The cadherin-catenin cell adhesion complex is the major building block of AJs, and has a crucial function in the dynamic behaviors of epithelial cells, such as cell polarization and cell rearrangements. The structure of α-catenin (100 kDa) consists of three distinct domains. The C-terminal actin-binding domain (ABD) (28 kDa), which is connected to the rest by a flexible P-linker region28 (2 kDa), directly binds to F-actin, and closely resembles the vinculin ABD (vin-ABD). The direct interaction between α-catenin and F-actin was demonstrated to be a catch bond, an interaction that is stabilized by increased force.

To better characterize the αE-catenin actin-binding site, we elucidated a crystal structure of αEcat-ABD-WT at 2.2-Å resolution. The electron density map of α5-helix clearly shows that V796 adopts a conformation that exposes its side chain on the ABD surface, along with two additional hydrophobic residues L785 and I792. Our observations of the cryptic (attenuated) and exposed (activated) conformations of V796, despite the nearly identical primary sequences of αEcat- and αNcat-ABDs (87% identity), indicate that this residue resides within a conformationally dynamic region. Consistent with this idea, the αEcat-ABD-WT structure contains an internal cavity that could accommodate V796 in the cryptic state similar to V796N in the αNcat-ABD-WT structure. This internal cavity is partly formed by the side chain of M673 from α1-helix, hence raising the possibility that α1-helix unfolding allosterically affects the F-actin-binding site by changing the conformational dynamics of V796. Our site-directed mutagenesis and actin cosedimentation assays with the αEcat-ABD variants support critical roles of these hydrophobic residues in F-actin-binding: Ala substitutions of L785, I792 and V796, individually or together as 3A, led to a range of reduction (75, 36, 47, and 78%, respectively) in the amount of ABD cosedimenting with F-actin compared to αEcat-ABD-WT. The equally significant reduction observed with either the L785A mutation alone or 3A suggests that L785 plays a central role in establishing the critical hydrophobic interface between F-actin and αcat-ABD. The measurable reduction in F-actin binding with I792A or V796A suggests that I792 and V796 are likely involved in further stabilizing this interface, and any changes to these residues could modulate the F-actin-binding activity of αcat-ABD. These results confirm that the hydrophobic residues on the α5-helix surface constitute an important binding surface for F-actin interaction.

>[2x]GPLGSPEFSRTSVQTEDDQLIAGQSARAIMAQLPQEQKAKIAEQVASFQEEKSKLDAEVSKWDDSGNDIIVLAKQMCMIMMEMTDFTRGKGPLKNTSDVISAAKKIAEAGSRMDKLGRTIADHCPDSACKQDLLAYLQRIALYCHQLNICSKVKAEVQNLGGELVVSGVDSAMSLIQAAKNLMNAVVQTVKASYVASTKYQKSQGMASLNLPAVSWKMKAPEKKPLVKREKQDETQTKIKRASQKKHVNPVQALSEFKAMDSI> LMVGGLLLAAASNNVQAEALQPDPAWQQGKLDNGFSWQLLATPQRPSDRIELRLIVNTGSLSENTQEVGFAHLLPRLALMSSASFTPAQLQSLWQQGIDNERPLPPAITSYDFTLYSLSLPNNRPDLLKDALAWLSDTAGNLAVSEQTVNAALNTATDPIATFPQNIQEPWWRYRLKGSSLIGHDPGQPVTQPVDVEKLKQFYQQWYTPDAMTLYVVGNVDSRSIAAQISKAFSELKGKRTAPAAVATLAPLPPEPVSLMNEQAAQDTLSLMWDTPWHPIQDSMALSRYWRSDLAREALFWHIKQVLEKNNQKNLKLGFDCRVQYQRAQCAIHLNTPVENLTANMTFVARELAALRANGLSQAEFDALMTQKNDQLSKLFATYARTDTDILMSQRLRSQQSGVVDIAPEQYQKLRQAFLSGLTLAELNRELKQQLSQDTTLVLMQPKGEPEVNVKALQEIYNGIMAPQTVAE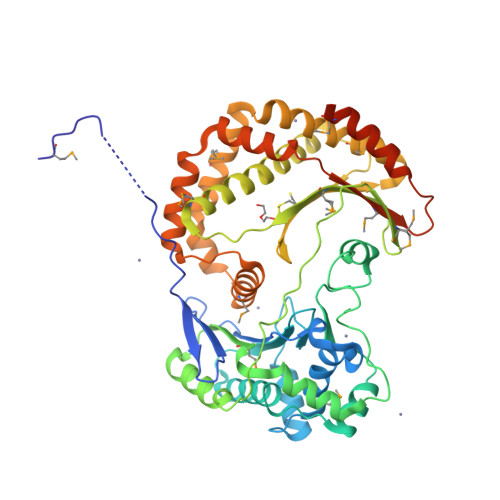EEVAPAEAVETAPVMPTTAQ> VTSVWTKGVTPPANFTQGEDVFHAPYVANQGWYDITKTFNGKDDLLCGAATAGNMLHWWFDQNKDQIKRYLEEHPEKQKINFNGEQMFDVKEAIDTKNHQLDSKLFEYFKEKAFPYLSTKHLGVFPDHVIDMFINGYRLSLTNHGPTPVKEGSKDPRGGIFDAVFTRGDQSKLLTSRHDFKEKNLKEISDLIKKELTEGKALGLSHTYANVRINHVINLWGADFDSNGNLKAIYVTDSDSNASIGMKKYFVGVNSAGKV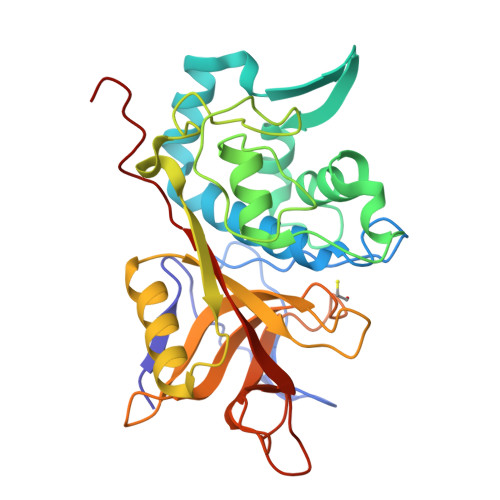AISAKEIKEDNIGAQVLGLFTLSTGQDSWNQTN N-[(4R)-6,8-dichloro-1,2,3,4-tetrahydroquinolin-4-yl]-N'-(5-fluoro-3H-imidazo[4,5-b]pyridin-2-yl)propane-1,3-diamine 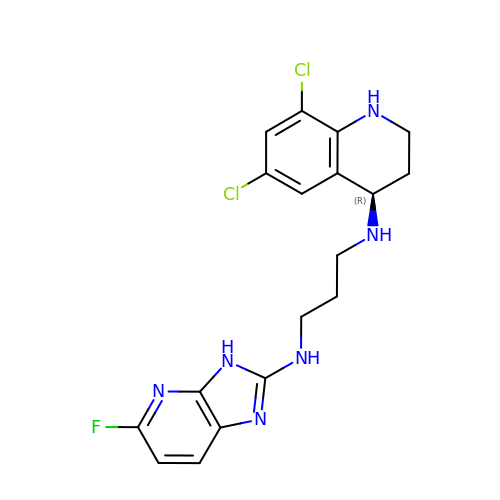| C18 H19 Cl2 F N6 | FPNBGOOGFIKSDR-CYBMUJFWSA-N> INQVRPKLPLLKILHAAGAQGEMFTVKEVMHYLGQYIMVKQLYDAAAQHMVYCGGDLLGELLGRQSFSVKD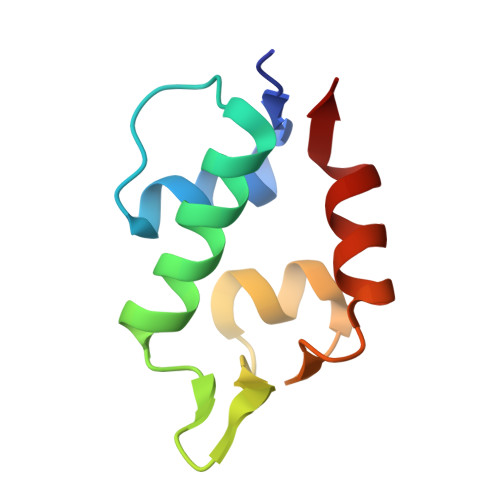PSPLYDMLRKNLVT>[2x]GMYTNTIIKTEIDEKVIKAFKLDA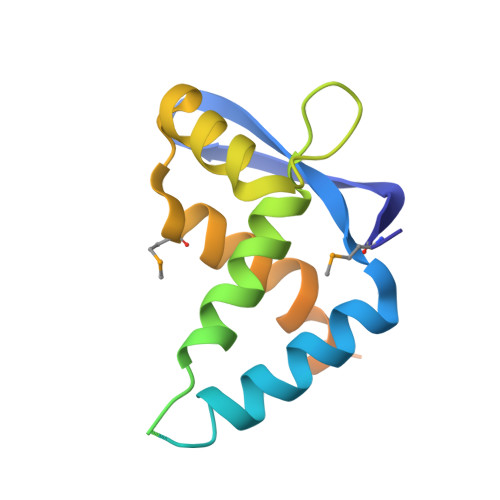LTRSKLFFKLTTKLAVPFAGVIDGAFSADRSLVSASVASLLSQHLDQETFEETQLILFGSIVEDGEALATPEAINKWFEYNDVNPMDLFVWLVDENLVTLFKGSKQLQSLKPKFDEFYKKFEDFIPQTVISDDKAEE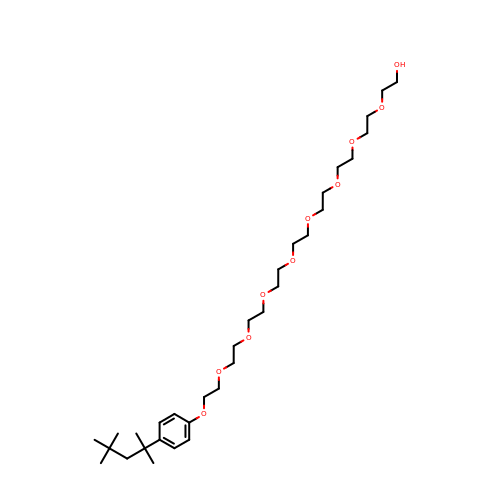2-(2-{2-[2-(2-{2-[2-(2-{2-[4-(1,1,3,3-TETRAMETHYL-BUTYL)-PHENOXY]-ETHOXY}-ETHOXY)-ETHOXY]-ETHOXY}-ETHOXY)-ETHOXY]-ETHOXY}-ETHOXY)-ETHANOL | C32 H58 O10 | VJYAJQFKKLYARJ-UHFFFAOYSA-N> MLVRLLRVILLASMVFCADILQLSYSDDAKDAIPLGTFEIDSTSDGNVTVTTVNIQDVEVSGEYCLNAQIEGKLDMPCFSYMKLRTPLKYDLIVDVDEDNEVKQVSLSYDETNDAITATVRYPEAGPTAPVTKLKKKTKTYADKKASKNKDGSTAQFEEDEEVKEVSWFQKNWKMLLLGLLIYNF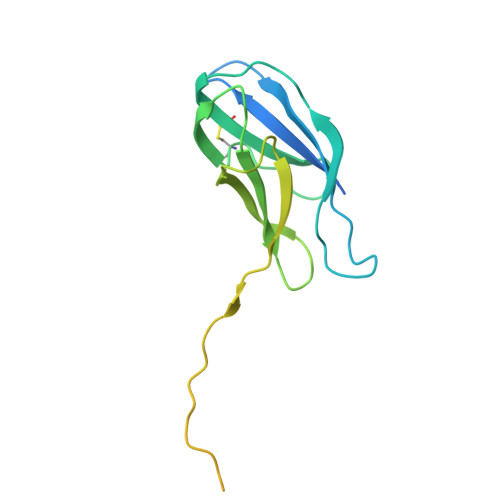VAGSAKKQQQGGAGADQKTE5'-O-(L-leucylsulfamoyl)adenosine | C16 H25 N7 O7 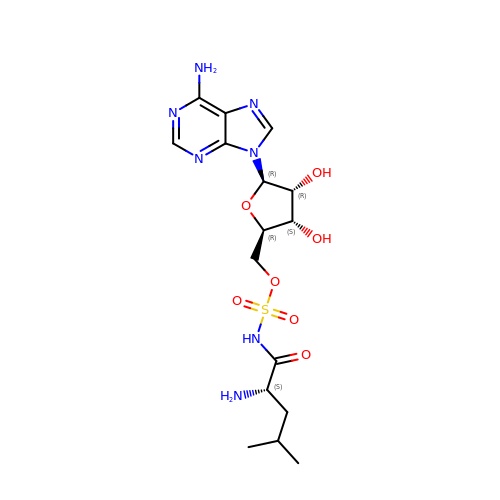S | XFEDFDTWJLGMBO-LEJQEAHTSA-N> MASGAPPSVDLTSIQWRMPEWVQSMGGLRTENVLEYFSQSPFYSHKSNNEMLKMQSQFNALDLGDLNSQL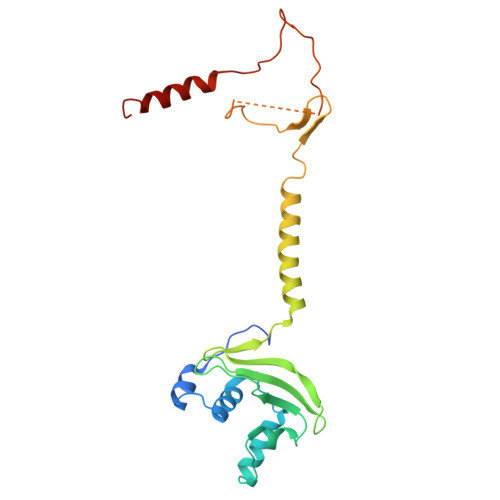KRLTGIQFVIIHERPPFLWVIQKQNRLNENEVKPLTVYFVCNENIYMAPNAYTLLATRMLNATYCFQKALTKIEKFPQYNPQEGYTYPKLSNDNLEVDHSNTNEPADENKNQSIENADYSFSPEDFSVVRAFMQSLHSSKEAPDVK>[2x]MTGPILSGLDPRFERTLYAHVGKEGSWTLDYYLRHGGYETAKRVLKEKTPDEVIEEVKRSGLRGRGGAGFPTGLKWSFMPKDDGKQHYLICNADESEPGSFKDRYILEDVPHLLIEGMILAGYAIRATVGYIYVRGEYRRAADRLEQAIKEARARGYLGKNLFGTDFSFDLHVHRGAGAYICGEETALMNSLEGLRANPRLKPPFPAQSGLWGKPTTINNVETLASVVPIMERGADWFAQMGTEQSKGMKLYQISGPVKRPGVYELPMGTTFRELIYEWAGGPLEPIQAIIPGGSSTPPLPFTEEVLDTPMSYEHLQAKGSMLGTGGVILIPERVSMVDAMWNLTRFYAHESCGKCTPCREGVAGFMVNLFAKIGTGQGEEKDVENLEALLPLIEGRSFCPLADAAVWPVKGSLRHFKDQYLALAREKRPVPRPSLWR;>[2x]MGFFDDKQDFLEETFAKYPPEGRRAAIMPLLRRVQQEEGWIRPERIEEIARLVGTTPTEVMGVASFYSYYQFVPTGKYHLQVCATLSCKLAGAEELWDYLTETLGIGPGEVTPDGLFSVQKVECLGSCHTAPVIQVNDEPYVECVTRARLEALLAGLRAGKRLEEIELPGKCGHHVHEVEV;>[2x]MVRVKVNDRIVEVPPGTSVMDAVFHAGYDVPLFCSEKHLSPIGACRMCLVRIGLPKKGPDGKPLLNEKGEPEIQWQPKLAASCVTAVADGMVVDTLSDVVREAQAGMVEFTLLNHPLDCPTCDKGGACELQDRTVEYGLYEKYYQKGPLELPVYTRFEFTRRHVDKHHPLSPFVILDRERCIHCKRCVRYFEEVPGDEVLDFIERGVHTFIGTMDFGLPSGFSGNITDICPVGALLDLTARFRARNWEMEETPTTCALCPVGCGITADTRSGELLRIRAREVPEVNEIWICDAGRFGHEWADQNRLKTPLVRKEGRLVEATWEEAFLALKEGLKEARGEEVGLYLAHDATLEEGLLASELAKALKTPHLDFQGRTAAPASLFPPASLEDLLQADFALVLGDPTEEAPILHLRLSEFVRDLKPPHRYNHGTPFADLQIKERMPRRTDKMALFAPYRAPLMKWAAIHEVHRPGEEREILLALLGDKEGSEMVAKAKEAWEKAKNPVLILGAGVLQDTVAAERARLLAERKGAKVLAMTPAANARGLEAMGVLPGAKGASWDEPGALYAYYGFVPPEEALKGKRFVVMHLSHLHPLAERYAHVVLPAPTFYEKRGHLVNLEGRVLPLSPAPIENGEAEGALQVLALLAEALGVRPPFRLHLEAQKALKARKVPEAMGRLSFRLKELRPKERKGAFYLRPTMWKAHQAVGKAQEAARAELWAHPETARAEALPEGAQVAVETPFGRVEARVVHREDVPKGHLYLSALGPAAGLRVEGRVLVPAGGEA;>[2x]MREEFLEEIPLDAPPEEAKELRTEVMTLNVGPQHPSTHGVLRLMVTLSGEEVLEVVPHIGYLHTGFEKTMEHRTYLQNITYTPRMDYLHSFAHDLAYALAVEKLLGAVVPPRAETIRVILNELSRLASHLVFLGTGLLDLGALTPFFYAFRERETILDLFEWVTGQRFHHNYIRIGGVKEDLPEEFVPELKKLLEVLPHRIDEYEALFAESPIFYERARGVGVIPPEVAIDLGLTGGSLRASGVNYDVRKAYPYSGYETYTFDVPLGERGDVFDRMLVRIREMRESVKIIKQALERLEPGPVRDPNPQITPPPRHLLETSMEAVIYHFKHYTEGFHPPKGEVYVPTESARGELGYYIVSDGGSMPYRVKVRAPSFVNLQSLPYACKGEQVPDMVAIIASLDPVMGDVDR;>MRLERVLEEARAKGYPIEDNGLGNLWVVLPRERFKEEMAHYKAMGFNFLADIVGLDYLTYPDPRPERFAVVYELVSLPGWKDGDGSRFFVRVYVPEEDPRLPTVTDLWGSANFLEREVYDLFGIVFEGHPDLRKILTPEDLEGHPLRKDYPLGETPTLFREGRYIIPAEFRAALTGKDPGLTFYKGGSRKGYRSLWADLKKAREVKG[2x];>[2x]MALKDLFERDVQELEREGILFTTLEKLVAWGRSNSLWPATFGLACCAIEMMASTDARNDLARFGSEVFRASPRQADVMIVAGRLSKKMAPVMRRVWEQMPDPKWVISMGACASSGGMFNNYAIVQNVDSVVPVDVYVPGCPPRPEALIYAVMQLQKKVRGQAYNERGERLPPVAAWKRTRG;>[2x]MSASSERELYEAWVELLSWMREYAQAKGVRFEKEADFPDFIYRMERPYDLPTTIMTASLSDGLGEPFLLADVSPRHAKLKRIGLRLPRAHIHLHAHYEPGKGLVTGKIPLTKERFFALADRAREALAFA;>[2x]MTLKALAQSLGITLKYLFSKPVTVPYPDAPVALKPRFHGRHVLTRHPNGLEKCIGCSLCAAACPAYAIYVEPAENDPENPVSAGERYAKVYEINMLRCIFCGLCEEACPTGAIVLGYDFEMADYEYSDLVYGKEDMLVDVVGTKPQRREAKRTGKPVKVGYVVPYVRPELEGFKAPTEGGKR;>MAPIQEYVGTLIYVGVALFIGVAALLVGALLGPKKPGRAKLMPYESGNDPAGEVKRFPVHFYVVAMLFILFDVEVAFLWPYAVSAG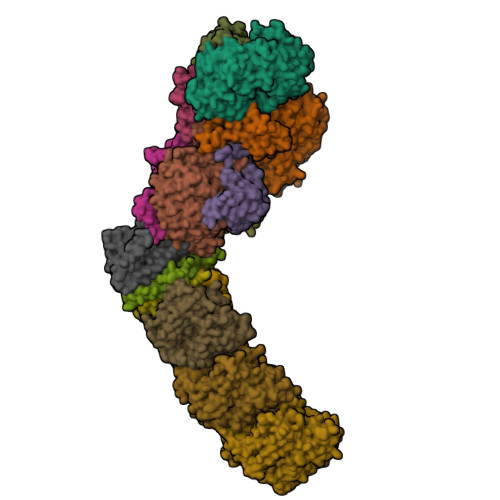GLGLYGFLGVLAFTLLLFVGFLYEWWKGVMRWH[2x];>MTWSYPVDPYWMVALKALLVVVGLLTAFAFMTLIERRLLARFQVRMGPNRVGPFGLLQPLADAIKSIFKEDIVVAQADRFLFVLAPLISVVFALLAFGLIPFGPPGSFFGYQPWVINLDLGILYLFAVSELAVYGIFLSGWASGSKYSLLGSLRSSASLISYELGLGLALLAPVLLVGSLNLNDIVNWQKEHGWLFLYAFPAFLVYLIASMAEAARTPFDLPEAEQELVGGYHTEYSSIKWALFQMAEYIHFITASALIPTLFLGGWTMPVLEVPYLWMFLKIAFFLFFFIWIRATWFRLRYDQLLRFGWGFLFPLALLWFLVTALVVALDLPRTYLLYLSALSFLVLLGAVLYTPKPARKGGGA[2x];>MSLLEGLALFLLLLSGVLVVTLRNAIHAALALILNFLVLAGVYVALDARFLGFIQVIVYAGAIVVLFLFVIMLLFAAQGEIGFDPLVRSRPLAALLALGVAGILAAGLWGLDLAFTQDLKGGLPQALGPLLYGDWLFVLLAVGFLLMAATVVAVALVEPGKASRAKEAEKREEVAR[2x];>MSYLLTSALLFALGVYGVLTRRTAILVFLSIELMLNAANLSLVGFARAYGLDGQVAALMVIAVAAAEVAVGLGLIVAIFRHRESTAVDDLSELRG[2x];>MALLGTILLPLLGFALLGLFGKRMREPLPGVLASGLVLASFLLGAGLLLSGGARFQAEWLPGIPFSLLLDNLSGFMLLIVTGVGFLIHVYAIGYMGGDPGYSRFFAYFNLFIAMMLTLVLADSYPVMFIGWEGVGLASFLLIGFWYKNPQYADSARKAFIVNRIGDLGFMLGMAILWALYGTLSISELKEAMEGPLKNPDLLALAGLLLFLGAVGKSAQIPLMVWLPDAMAGPTPVSALIHAATMVTAGVYLIARSSFLYSVLPDVSYAIAVVGLLTAAYGALSAFGQTDIKKIVAYSTISQLGYMFLAAGVGAYWVALFHVFTHAFFKALLFLASGSVIHALGGEQDVRKMGGLWKHLPQTRWHALIGALALGGLPLLSGFWSKDAILAATLTYPFGGVGFYVGALLVAVLTAMYAMRWFVLVFLGEERGHHHPHEAPPVMLWPNHLLALGSVLAGYLALPHPLPNVLEPFLKPALAEVEAHHLSLGAEWGLIALSAAVALLGLWAGFVFFQRKVFPAWYLAFEAASREAFYVDRAYNALIVNPLKALAEALFYGDRGLLSGYFGLGGAARSLGQGLARLQTGYLRVYALLFVLGALLLLGVMRW[2x];>[2x]MVVLAVLLPVVFGALLLLGLPRALGVLGAGLSFLLNLYLFLTHPGGVAHAFQAPLLPGAGVYWAFGLDGLSALFFLTIALTVFLGALVARVEGRFLGLALLMEGLLLGLFAARDLLVFYVFFEAALIPALLMLYLYGGEGRTRALYTFVLFTLVGSLPMLAAVLGARLLSGSPTFLLEDLLAHPLQEEAAFWVFLGFALAFAIKTPLFPLHAWLPPFHQENHPSGLADALGTLYKVGVFAFFRFAIPLAPEGFAQAQGLLLFLAALSALYGAWVAFAAKDFKTLLAYAGLSHMGVAALGVFSGTPEGAMGGLYLLAASGVYTGGLFLLAGRLYERTGTLEIGRYRGLAQSAPGLAALALILFLAMVGLPGLSGFPGEFLTLLGAYKASPWLAALAFLSVIASAAYALTAFQKTFWEEGGSGVKDLAGAEWGFALLSVLALLLMGVFPGYFARGLHPLAEAFAKLLGGGA;>[2x]MTLAILAVFSVALTLLGFVLPPQGVKRATLLGLALALASLLLTWGKPFAFGPYAVDGVSQVFTLLALLGALWTVGLVRSGRFEFYLLVLYAALGMHLLASTRHLLLMLVALEALSLPLYALATWRRGQGLEAALKYFLLGALAAAFFLYGAALFYGATGSLVLGAPGEGPLYALALGLLLVGLGFKAALAPFHFWTPDVYQGSPTPVVLFMATSVKAAAFAALLRVAAPPEALALLVALSVVVGNLAALAQKEAKRLLAYSSIAHAGYMALALYTGNAQALGFYLLTYVLATGLAFAVLSQISPDRVPLEALRGLYRKDPLLGLAFLVAMLSLLGLPPLAGFWGKYLAFAEAARAGAWGVLVLALVTSAVSAYYYLGLGLAVFARPEETPFRPGPPWARAAVVAAGVLLLALGLLPGLVLPALAAGG;>MVRVGMRAAPRVSLEALKAALGGLKLSEAKVYLITDWQDKRDQARYALLLHTGKKDLLVPDAFGPAFPGGEEALSELVGLLLAQGARRFYEAVVSPGEMTALLDLPPEELLKRVMAIANPTDPGIYLKRAA[2x]> MASSNLIKQLQERGLVAQVTDEEALAERLAQGPIALYCGFDPTADSLHLGHLVPLLCLKRFQQAGHKPVALVGGATGLIGDPSF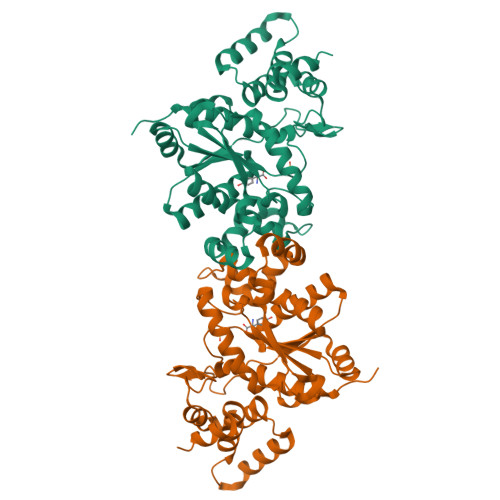KAAERKLNTEETVQEWVDKIRKQVAPFLDFDCGENSAIAANNYDWFGNMNVLTFLRDIGKHFSVNQMINKEAVKQRLNREDQGISFTEFSYNLLQGYDFACLNKQYGVVLQIGGSDQWGNITSGIDLTRRLHQNQVFGLTVPLITKADGTKFGKTEGGAVWLDPKKTSPYKFYQFWINTADADVYRFLKFFTFMSIEEINALEEEDKNSGKAPRAQYVLAEQVTRLVHGEEGLQAAKR>[6x]STIPSEIINWTILNEIISMDDDDSDFSKGLIIQFIDQAQTTFAQMQRQLDGEKNLTELDNLGHFLKGSSAALGLQRIAWVCERIQNLGRKMEHFFPNKTELVNTLSDKSIINGIN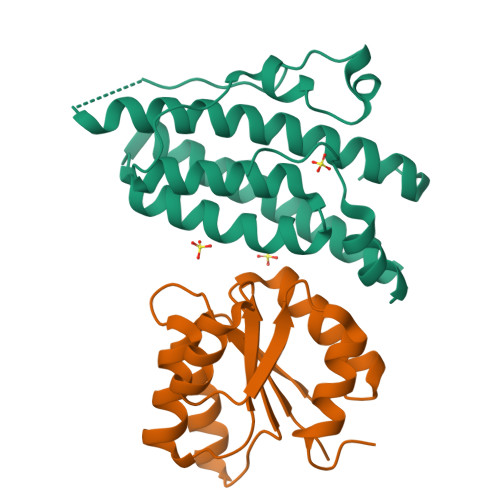IDEDDEEIKIQVDDKDENSIYLILIAKALNQSRLEFKLARIELSKYYNTNL;>[6x]SVKILVVEDNHVNQEVIKRMLNLEGIENIELACDGQEAFDKVKELTSKGENYNMIFMDVQMPKVDGLLSTKMIRRDLGYTSPIVALTAFADDSNIKECLESGMNGFLSKPIKRPKLKTILTEFCAAYQGKKNNK>[6x]MRGSHHHHHHTDPLDVDSEPDVSAKMAGRSMQAARCPTDELSLSNCAVVSEKDYQSGQHVIVRTSPNHKYIFTLRTHPSVVPGSVAFSLPQRKWAGLSIGQEIEVALYSFDKAKQCIGTMTIEIDFLQKKNIDSNPYDTDKMAAEFIQQFNNQAFSVGQQLVFSFNDKLFGLLVKDIEAVDPSILKGEPASGKRQKIEVGLV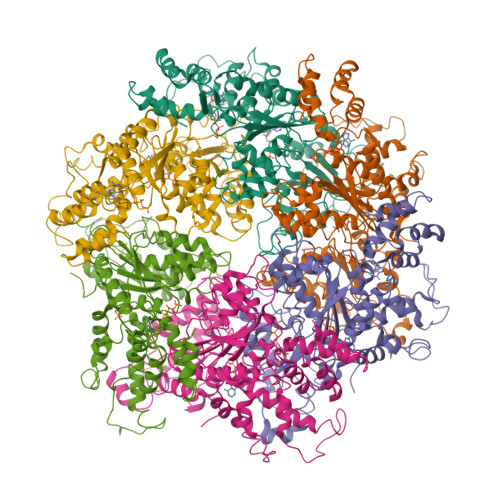VGNSQVAFEKAENSSLNLIGKAKTKENRQSIINPDWNFEKMGIGGLDKEFSDIFRRAFASRVFPPEIVEQMGCKHVKGILLYGPPGCGKTLLARQIGKMLNAREPKVVNGPEILNKYVGESEANIRKLFADAEEEQRRLGANSGLHIIIFDEIDAICKQRGSMAGSTGVHDTVVNQLLSKIDGVEQLNNILVIGMTNRPDLIDEALLRPGRLEVKMEIGLPDEKGRLQILHIHTARMRGHQLLSADVDIKELAVETKNFSGAELEGLVRAAQSTAMNRHIKASTKVEVDMEKAESLQVTRGDFLASLENDIKPAFGTNQEDYASYIMNGIIKWGDPVTRVLDDGELLVQQTKNSDRTPLVSVLLEGPPHSGKTALAAKIAEESNFPFIKICSPDKMIGFSETAKCQAMKKIFDDAYKSQLSCVVVDDIERLLDYVPIGPRFSNLVLQALLVLLKKAPPQGRKLLIIGTTSRKDVLQEMEMLNAFSTTIHVPNIATGEQLLEALELLGNFKDKERTTIAQQVKGKKVWIGIKKLLMLIEMSLQMDPEYRVRKFLALLREEGASPLDFD>EDPLAKKQTVRLIKDLQRAINKVLCTRLRLSNFFTIDHFIQKLHTARKILVLTGAGVSTSLGIPDFRSSEGFYSKIKHLGLDDPQDVFNYNIFMHDPSVFYNIANMVLPPEKIYSPLHSFIKMLQMKGKLLRNYTQNIDNLESYAGISTDKLVQCHGSFATATCVTCHWNLPGERIFNKIRNLELPLCPYCYKKRREYFPEGYNNKVGVAASQGSMSERPPYILNSYGVLKPDITFFGEALPNKFHKSIREDILECDLLICIGTSLKVAPVSEIVNMVPSHVPQVLINRDPVKHAEFDLSLLGYCDDIAAMVAQKCGWTIPHKKWNDLKNKNFKCQEKDKGVYVVTSDEHPKTL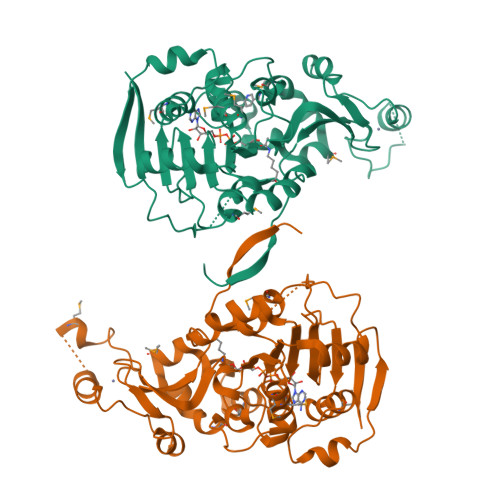[2x]> MTDNPNKKTFWDKVHLDPTMLLILLALLVYSALVIWSASGQDIGMMERKIGQIAMGLVIMVVMAQIPPRVYEGWAPYLYIICIILLVAVDAFGAISKGAQRWLDLGIVRFQPSEIAKIAVPLMVARFINRDVCPPSLKNTGIALVLIFMPTLLVAAQPDLGTSILVALSGLFVLFLSGLSWRLIGVAVVLVAAFIPILWFFLMHDYQRQRVMMLLDPESDPLGAGYHIIQSKIAIGSGGLRGKGWLHGTQSQLEFLPERHTDFIFAVLAEELGLVGILILLALYILLIMRGLWIAARAQTTFGRVMAGGLMLILFVYVFVNIGMVSGILPVVGVPLPLVSYGGSALIVLMAGFGIVMSIHTHRKMLSKSV;> MKLQNSFRDYTAESALFVRRALVAFLGILLLTGVLIANLYNLQIVRFTDYQTRSNENRIKLVPIAPSRGIIYDRNGIPLALNRTIYQIEMMPEKVDNVQQTLDALRSVVDLTDDDIAAFRKERARSHRFTSIPVKTNLTEVQVARFAVNQYRFPGVEVKGYKRRYYPYGSALTHVIGYVSKINDKDVERLNNDGKLANYAATHDIGKLGIERYYEDVLHGQTGYEEVEVNNRGRVIRQLKEVPPQAGHDIYLTLDLKLQQYIETLLAGSRAAVVVTDPRTGGVLALVSTPSYDPNLFVDGISSKDYSALLNDPNTPLVNRATQGVYPPASTVKPYVAVSALSAGV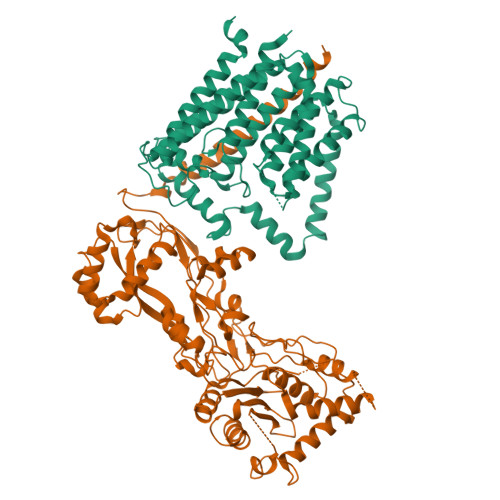ITRNTTLFDPGWWQLPGSEKRYRDWKKWGHGRLNVTRSLEESADTFFYQVAYDMGIDRLSEWMGKFGYGHYTGIDLAEERSGNMPTREWKQKRFKKPWYQGDTIPVGIGQGYWTATPIQMSKALMILINDGIVKVPHLLMSTAEDGKQVPWVQPHEPPVGDIHSGYWELAKDGMYGVANRPNGTAHKYFASAPYKIAAKSGTAQVFGLKANETYNAHKIAERLRDHKLMTAFAPYNNPQVAVAMILENGGAGPAVGTLMRQILDHIMLGDNNTDLPAENPAVAAAEDH> MLAGVKKDIEKLYEAVPQLSNVFKIEDKIGEGTFSSVYLATAQLQVGPEEKIALKHLIPTSHPIRIAAELQCLTVAGGQDNVMGVKYCFRKNDHVVIAMPYLEHESFLDILNSLSFQEVREYMLNLFKALKRIHQFGIVHRDVKPSNFLYNRRLKKYALVD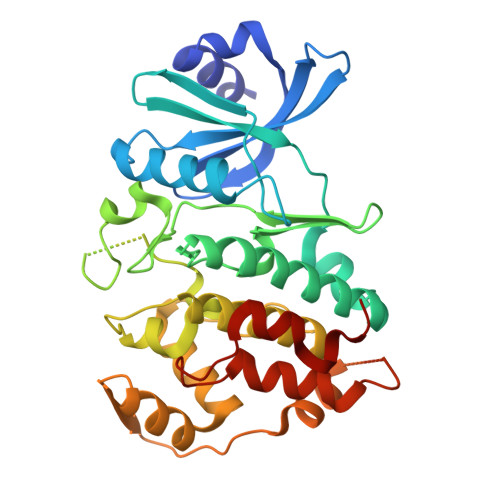FGLAQGTHDTKIELLKFVQSEAQQERCSQNKCSICLSRRQQVAPRAGTPGFRAPEVLTKCPNQTTAIDMWSAGVIFLSLLSGRYPFYKASDDLTALAQIMTIRGSRETIQAAKTFGKSILCSKEVPAQDLRKLCERLRGMDSSTPKLTSDIQGHATNLEGWNEVPDEAYDLLDKLLDLNPASRITAEEALLHPFFKDMSL>[2x]SVYTYFSAVAGQDGEVDAEELQRCLTQSGINGTYSPFSLETCRIMIA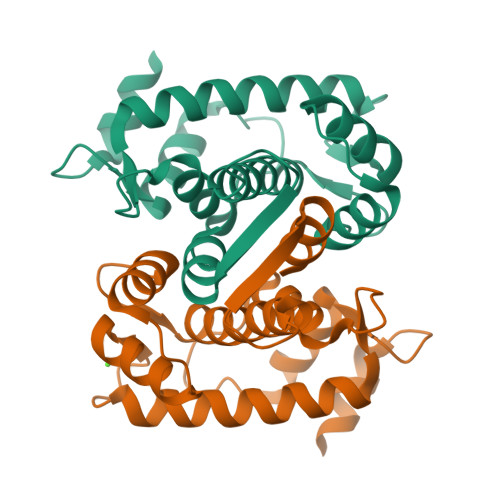MLDRDHTGKMGFNAFKELWAALNAWKENFMTVDQDGSGTVEHHELRQAIGLMGYRLSPQTLTTIVKRYSKNGRIFFDDYVACCVKLRALTDFFKKRDHLQQGSADFIYDDFLQGTMAI>MAHHHHHHMVHITLDPDTANPWLILSEDRRQVRLGDTQQSIPGNEERFDSYPMVLGAQHFHSGKHYWEVDVTGKEAWDLGVCRDSVRRKGHFLLSSKSGFWTIWLWNKQKYEAGTYPQTPLHLQVPPCQVGIFLDYEAGMVSFYNITDHGSLIYSFSECAFTGPLRPFFSPGFNDGGKNT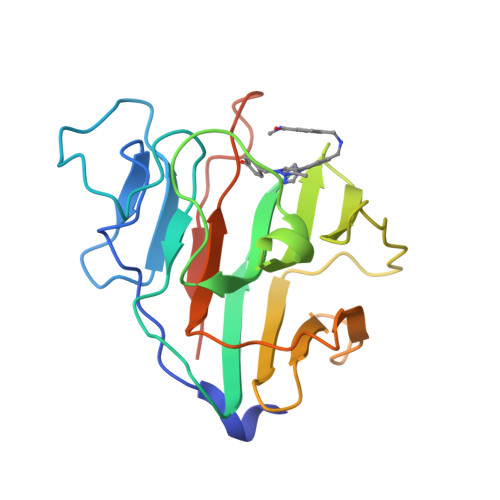APLTLCPLNIGSQGSTDY[4x]phenyl ethenesulfonate | C8 H8 O3 S | 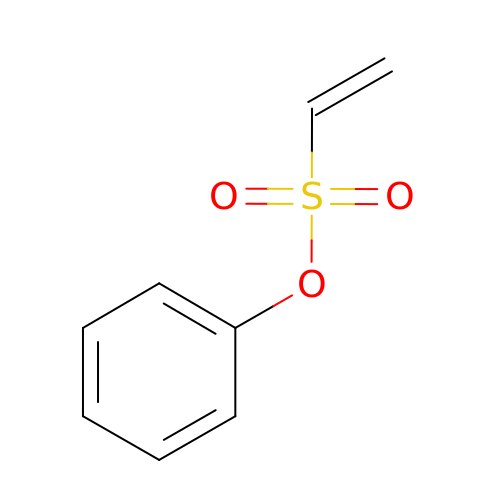CILDJVVXNMDAGY-UHFFFAOYSA-N> AEIYNKDGNKVDLYGKAVGLHYFSKGNGENSYGGNGDMTYARLGFKGETQINSDLTGYGQWEYNFQGNNSEGAAAQTGNKTRLAFAGLKYADVGSFDYGRNYGVVYDALGYTDMLPEFGGDTAYSDDFFVGRVGGVATYRNSNFFGLVDGLNFAVQYLGKNERDTARRSNGDGVGGSISYEYEGFGIVGAYGAADRTNLQEAQPLGNGKKAEQWATGLKYDANNIYLAANYGETRNATPITNKFTNTSGFANKTQ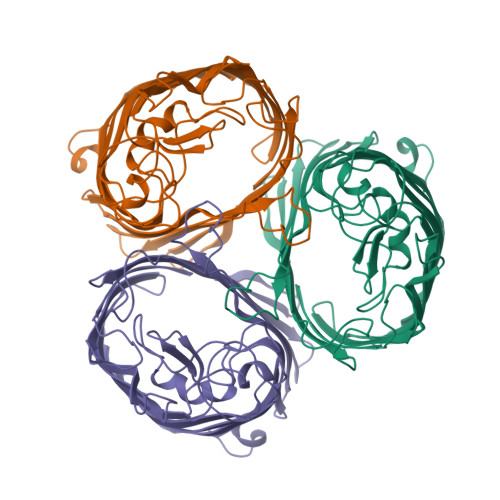DVLLVAQYQFDFGLRPSIAYTKSKAKDVEGIGDVDLVNYFEVGATYYFNKNMSTYVDYIINQIDSDNKLGVGSDDTVAVGIVYQF> SMGKLSEQLKHCNG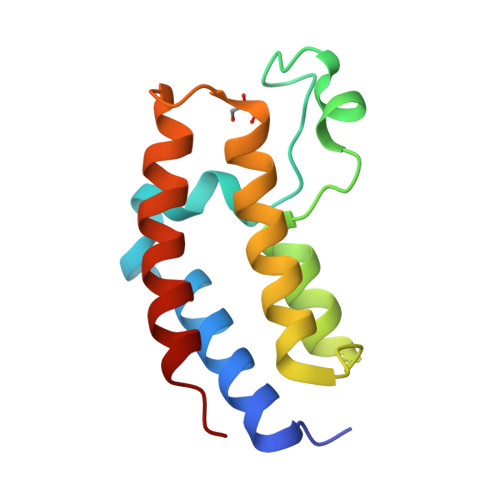ILKELLSKKHAAYAWPFYKPVDASALGAHDYHDIIKHPMDLSTVKRKMENRDYRDAQEFAADVRLMFSNCYKYNPPDHDVVAMARKLQDVFEFRYAKMPD RAR-Related Orphan Receptor C (RORγ, gene name RORC) is an orphan nuclear receptor (NR) that is widely expressed and is involved in regulation of various metabolic processes. RORγ is also a key player in the immune system where the lymphocyte specific isoform RORγt is a so-called ‘master regulator’ of the IL-17 producing T helper (Th17) cell subset. Structural and functional analysis has revealed that the RORγ ligand binding domain (RORγLBD) is comprised of 12 α-helices (H1-H12) and a β-sheet region (BSR) that responds to cholesterol biosynthetic pathway intermediates, hydroxysterols and sterol sulfates. The results presented here indicate that the RORγLBD requires a ligand to stabilize the active conformer and that hyperactivating ligands enhance coactivator affinities by allosterically driving electrostatic intramolecular interactions between H12 and H4.

After obtaining co-crystal structures of partial agonist SR19265 and antagonist SR19355, we attempted and failed to solve co-crystal structures of full agonist SR19547 bound to the RORγLBD. While most compounds protected H12, SR19269 and SR19355 exhibited little protection to this region. However, SR19355 and SR19269 also exhibit commensurate H4 protection showing that the observed H4 stability depends on H12 stability. Importantly, SR19355 displayed much higher performance in this assay with no commensurate increase in protection at these regions. This highlights an important limitation to the approach where differences in binding mode (an additional hydrogen bond in this case) can identify compounds as outliers.

> ASLTEIEHLVQSVCKSYRETCQLRLEDLLRQRSNIFSREEVTGYQRKSMWEMWERCAHHLTEAIQYVVEFAKRLSGFMELCQNDQIVLLKAGAMEVVLVRMCRAYNADNRTVFFEGKYGGMELFRALGCSELISSIFDFSHSLSALHFSEDEIALYTALVLINAHRPGLQEKRKVEQLQYNLELAFHHHLCKTHRQSILAKLPPKGKLRSLCSQHVERLQIFQHLHPIVVQAAFPPLYKELFSGGGEKHKILHRLLQDS> MPVTINNFNYNDPIDNNNIIMMEPPFARGTGRYYKAFKITDRIWIIPERYTFGYKPEDFNKSSGIFNRDVCEYYDPDYLNTNDKKNIFLQTMIKLFNRIKSKPLGEKLLEMIINGIPYLGDRRVPLEEFNTNIASVTVNKLISNPGEVERKKGIFANLIIFGPGPVLNENETIDIGIQNHFASREGFGGIMQMKFCPEYVSVFNNVQENKGASIFNRRGYFSDPALILMHELIHVLHGLYGIKVDDLPIVPNEKKFFMQSTDAIQAEELYTFGGQDPSIITPSTDKSIYDKVLQNFRGIVDRLNKVLVCISDPNININIYKNKFKDKYKFVEDSEGKYSIDVESFDKLYKSLMFGFTETNIAENYKIKTRASYFSDSLPPVKIKNLLDNEIYTIEEGFNISDKDMEKEYRGQNKAINKQAYEEISKEHLAVYKIQMCVDGGGGSGGGGSGGGGSAIEGRAGGGGSGGGGSGGGGSALVLQCIDVDNEDLFFIADKNSFSDDLSKNERIEYNTQSNYIENDFPINELILDTDLISKIELPSENTESLTDFNVDVPVYEKQPAIKKIFTDENTIFQYLYSQTFPLDIRDISLTSSFDDALLFSNKVYSFFSMDYIKTANKVVEAGLFAGWVKQIVNDFVIEANKSNTMDKIADISLIVPYIGLALNVGNETAKGNFENAFEIAGASILLEFIPELLIPVVGAFLLESYIDNKNKIIKTIDNALTKRNEKWSDMYGLIVAQWLSTVNTQFYTIKEGMYKALNYQAQALEEIIK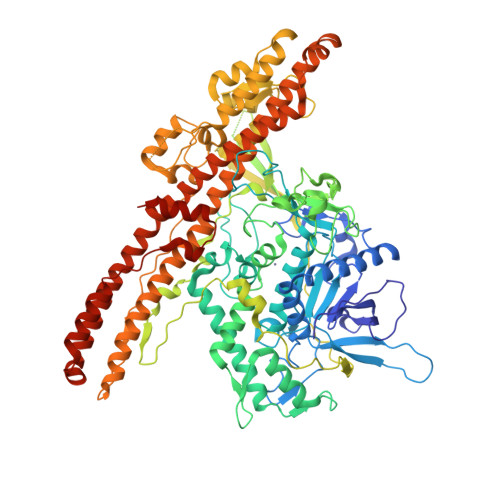YRYNIYSEKEKSNINIDFNDINSKLNEGINQAIDNINNFINGCSVSYLMKKMIPLAVEKLLDFDNTLKKNLLNYIDENKLYLIGSAEYEKSKVNKYLKTIMPFDLSIYTNDTILIEMFNKYNSLEALASGHHHHHH> SNASERTGTQPLGVQGLTEEQRMMIRELMDAQMKTFDTTFSHFKNFRLPGVLSSGCELPESLQAPSREEAAKWSQVRKDLCSLKVSLQLRGEDGSVWNYKPPADSGGKEIFSLLPHMADMSTYMFKGIISFAKVISYFRDLPIEDQISLLKGAAFELCQLRFNTVFNAETGTWECGRLSYCLEDTAGGFQQLLLEPMLKFH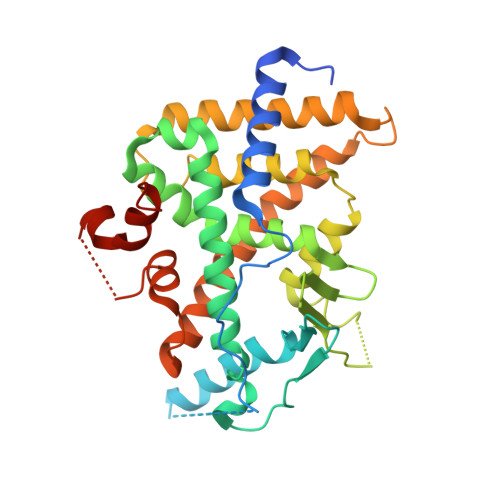YMLKKLQLHEEEYVLMQAISLFSPDRPGVLQHRVVDQLQEQFAITLKSYIECNRPQPAHRFLFLKIMAMLTELRSINAQHTQRLLRIQDIHPFATPLMQELFGITGSGGSGGSSHSSLTERHKILHRLLQEGSPS>MGHHHHHHHHHHSSGHIDDDDKHMEVKQENRLLNESESSSQGLLGYYFSDLNFQAPMVVTSSTTGDLSIPSSELENIPSENQYFQSAIWSGFIKVKKSDEYTFATSADNHVTMWVDDQEVINKASNSNKIRLEKGRLYQIKIQYQRENPTEKGLDFKLYWTDSQNKKEVISSDNLQLPELKQKSSNSRKKRSTSAGPTVPDRDNDGIPDSLEVEGYTVDVKNKRTFLSPWISNIHEKKGLTKYKSSPEKWSTASDPYSDFEKVTGRIDKNVSPEARHPLVAAYPIVHVDMENIILSKNEDQSTQNTDSQTRTISKNTSTSRTHTSEVHGNAEVHASFFDIGGSVSAGFSNSNSSTVAIDHSLSLAGERTWAETMGLNTADTARLNANIRYVNTGTAPIYNVLPTTSLVLGKNQTLATIKAKENQLSQILAPNNYYPSKNLAPIALNAQDDFSSTPITMNYNQFLELEKTKQLRLDTDQVYGNIATYNFENGRVRVDTGSNWSEVLPQIQETTARIIFNGKDLNLVERRIAAVNPSDPLETTKPDMTLKEALKIAFGFNEPNGNLQYQGKDITEFDFNFDQQTSQNIKNQLAELNATNIYTVLDKIKLNAKMNILIRDKRFHYDRNNIAVGADESVVKEAHREVINSSTEGLLLNIDKDIRKILSGYIVEIEDTEGLKEVINDRYDMLNISSLRQDGKTFIDFKKYNDKLPLYISNPNYKVNVYAVTKENTIINPSENGDTSTNGIKKILIFSKKGYEIG[7x];>[3x]MNIKKEFIKVISMSCLVTAITLSGPVFIPLVQGAGGHGDVGMHVKEKEKNKDENKRKDEERNKTQEEHLKEIMKHIVKIEVKGEEAVKKEAAEKLLEKVPSDVLEMYKAIGGKIYIVDGDITKHISLEALSEDKKKIKDIYGKDALLHEHYVYAKEGYEPVLVIQSSEDYVENTEKALNVYYEIGKILSRDILSKINQPYQKFLDVLNTIKNASDSDGQDLLFTNQLKEHPTDFSVEFLEQNSNEVQEVFAKAFAYYIEPQHRDVLQLYAPEAFNYMDKFNEQEINLSLEELKDQRMLARYEKWEKIKQHYQHWSDSLSEEGRGLLKKLQIPIEPKKDDIIHSLSQEEKELLKRIQIDSSDFLSTEEKEFLKKLQIDIRDSLSEEEKELLNRIQVDSSNPLSEKEKEFLKKLKLDIQPYDINQRLQDTGGLIDSPSINLDVRKQYKRDIQNIDALLHQSIGSTLYNKIYLYENMNINNLTATLGADLVDSTDNTKINRGIFNEFKKNFKYSISSNYMIVDINERPALDNERLKWRIQLSPDTRAGYLENGKLILQRNIGLEIKDVQIIKQSEKEYIRIDAKVVPKSKIDTKIQEAQLNINQEWNKALGLPKYTKLITFNVHNRYASNIVESAYLILNEWKNNIQSDLIKKVTNYL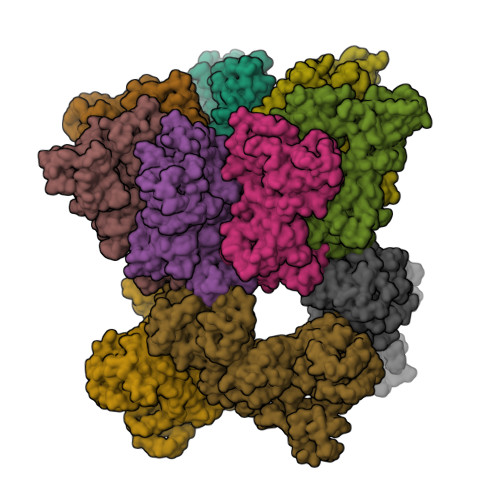VDGNGRFVFTDITLPNIAEQYTHQDEIYEQVHSKGLYVPESRSILLHGPSKGVELRNDSEGFIHEFGHAVDDYAGYLLDKNQSDLVTNSKKFIDIFKEEGSNLTSYGRTNEAEFFAEAFRLMHSTDHAERLKVQKNAPKTFQFINDQIKFIINS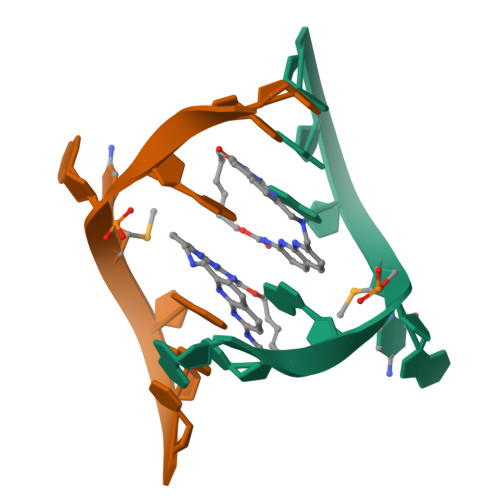>GCAGCAGC[2x]>[4x]MIAYHTLTKALLFPDIDQYQHWHHVAPMLAKMLVDGKYSIHQQYEYLCLFAQLVAPVLGPYPSPGRDVYRCTLGGNMTVELSQNFQRSGSTTRIAFEPVRYQASVGHDRFNRTSVNAFFSQLQLLVKSVNIELHHLLSEHLTLTAKDER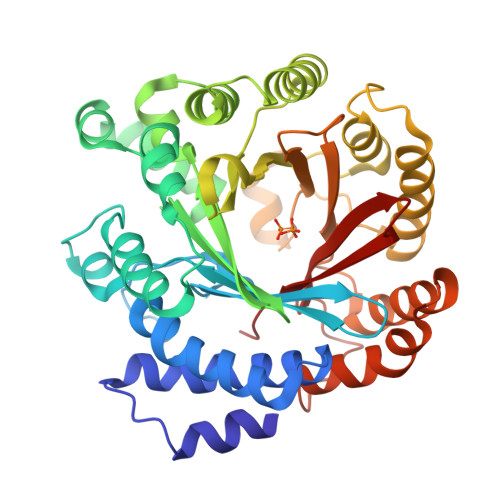NLNEEQLTKYLTNFQVKTQYVVALDLRKTGIVAKEYFFPGIKCAATGQTGSNACFGAIRAVDKDGHLDSLCQLIEAHFQQSKIDDAFLCCDLVDPAHTRFKVYIADPLVTLARAEEHWTLGGRLTDEDAAVGLEIIRGLWSELGIIQGPLEPSAMMEKGLLPIMLNYEMKAGQRLPKPKLYMPLTGIPETKIARIMTAFFQRHDMPEQAEVFMENLQAYYEGKNLEEATRYQAWLSFAYTKEKGPYLSIYYFWPE>GLKEQLASMNAIANVKATYSINGETFQIPSSDIMSWLTYNDGKVDLDTE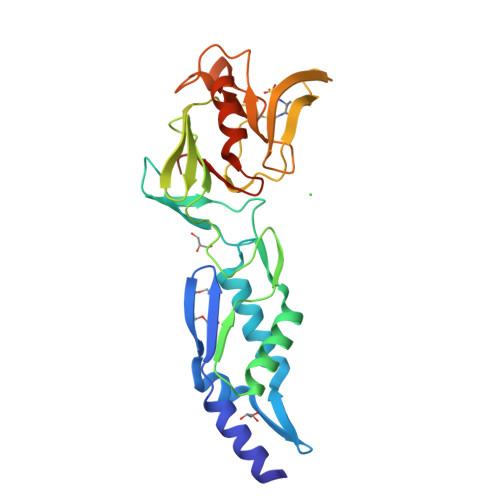QVRQYVTDLGTKYNTSTNDTKFKSTKRGEVTVPVGTYSWTIQTDSETEALKKAILAGQDFTRSPIVQGGTTADHPLIEDTYIEVDLENQHMWYYKDGKVALETDIVSGKPTTPTPAGVFYVWNKEEDATLKGTNGTPYESPVNYWMPIDWTGVGIHDSDWQPEYGGDLWKTRGSHGCINTPPSVMKELFGMVEKGTPVLVFGSHHHHHH[3x]>[4x]MKRKIIFLASPY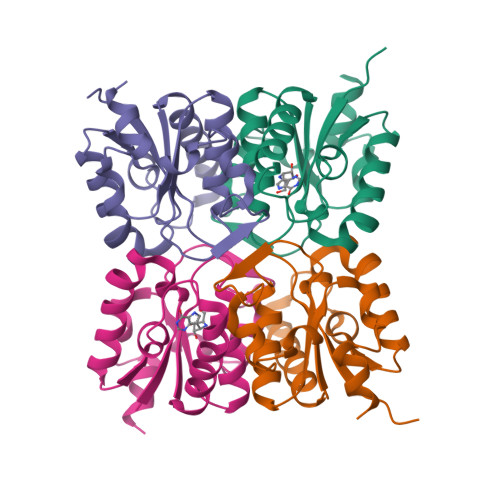GFSQQQKTLLLPPIVRALEALGIEVWEPFARNNQIDFSQADWAYRVAQADLQDVKNCDGIFAVVNGTPPDEGVMVELGMAIALNKAIFLFRDDFRRCSDNERYPLNLMLFAGLPEIGWENYYYTSVDEIQSHDKALYKWLTG> KPCCDQCACTKSNPPQCRCSDMRLNSCHSACKSCICALSYPAQCFCVDI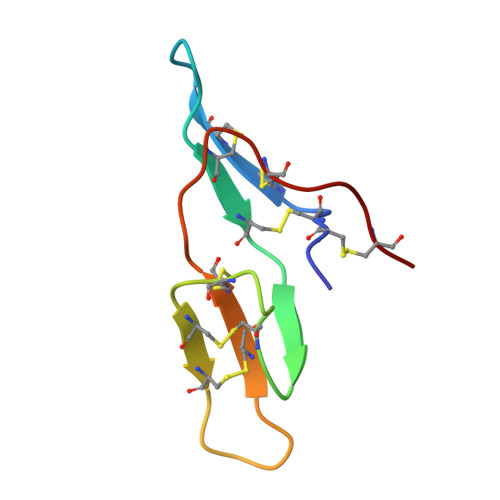TDFCYEPCK>[2x]GHHHHHHHGESLFKGPRDYNPISSTICHLTNESDGHTTSLYGIGFGPFIITNKHLFRRNNGTLLVQSLHGVFKVKNTTTLQQHLIDGRDMIIIRMPKDFPPFPQKLKFREPQREERICLVTTNFQTKSMSSMVSDTSCT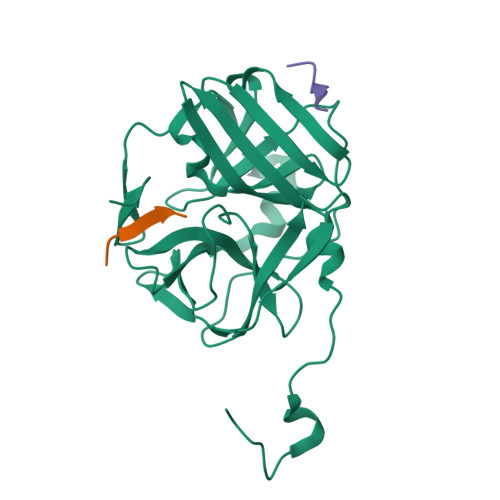FPSSDGIFWKHWIQTKDGQCGSPLVSTRDGFIVGIHSASNFTNTNNYFTSVPKNFMELLTNQEAQQWVSGWRLNADSVLWGGHKVFMDKP;>[2x]XENLYFQSGT;> EATQLMN>[2x]SNAMHMLRIAKEALT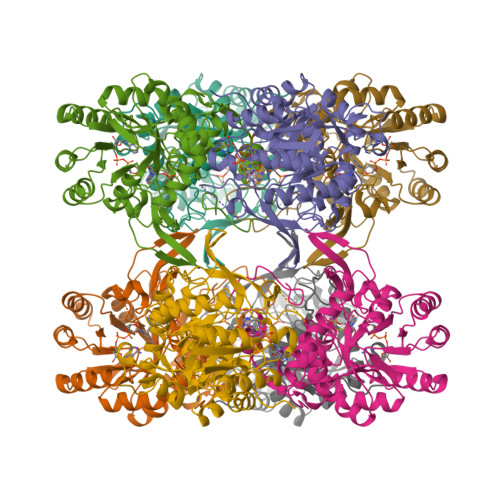FDDVLLVPAHSTVLPNTADLRTRLTKNIALNIPMVSASMDTVTEARLAIALAQEGGIGFIHKNMSIEQQAAQVHQVKISGGLRVGAAVGAAPGNEERVKALVEAGVDVLLIDSSHGHSEGVLQRIRETRAAYPHLEIIGGNVATAEGARALIEAGVSAVKVGIGPGSICTTRIVTGVGVPQITAIADAAGVANEYGIPVIADGGIRFSGDISKAIAAGASCVMVGSMFAGTEEAPGEVILYQGRSYKAYRGMGSLGAMSKGSSDRYFQTDNAADKLVPEGIEGRIAYKGHLKEIIHQQMGGLRSCMGLTGSATVEDLRTKAQFVRISGAGMKESHVHDVQITKEAPNYRLG Microfibril-associated glycoprotein 4 (MFAP4) is a 36 kDa extracellular matrix glycoprotein present in elastic fibre-rich tissues. MFAP4 consists of an N-terminal signal peptide, an RGD recognition site for cell surface integrin receptors, and a C-terminal fibrinogen-related domain (FReD), which constitutes the bulk of the protein. MFAP4 partakes in elastin fibre formation (elastogenesis) and in extracellular matrix organisation by protein-protein and cell-matrix interactions. MFAP4 multimerises and interacts with elastogenic proteins, including fibrillin-1 and tropoelastin, and with cells via integrins.

The presented 2D classes were collectively used for initial reference generation and subsequent 3D reconstruction using C1 point group symmetry, confirming that MFAP4 organizes as an octameric structure. Further refinement of the 3D cryo-EM map with D2 symmetry produced a 3.55 Å resolution (masked Fourier shell correlation (FSC)half-map = 0.143, Supplementary Figs. 2 and 3) structure of octameric MFAP4. Thus, the top and bottom halves of the MFAP4 octamer, defined across the central XY plane, can be described as two tetramers, each composed of two dimers with N-termini linked by C34 disulphide bonds. Within the tetrameric top and bottom halves of the MFAP4 octamer, monomers interact through intra-tetrameric interfaces, including potential salt-bridge interactions between interchain residues R105-D159 and R94-E158, hydrogen bonds between interchain residues A106-N152, G104-E158, G104-V154, and R94-E158, as well as non-bonded interchain interactions between R105-N152, G104-D159 and F103-E158. The top and bottom halves of the MFAP4 octamer associate through inter-tetrameric interfaces, including a polar non-bonded interchain interaction between N231-A200 and non-polar non-bonded interchain interactions between V196-F93, L202-L202, S204-L202. Between tetrameric halves of the MFAP4 octamer, the buried solvent-accessible surface area is 433 Å2 and is shared between 22 contacting residues (13 residues from each adjacent chain). Although the N-termini preceding Q37 are not resolved within the map model and are predicted to be disordered regions by AlphaFold2, we observed that the Q37 residues of each of the four MFAP4 molecules at the top and bottom of an octamer are positioned to extend towards each other and outwards from the macromolecular assembly. This arrangement potentially positions four integrin-binding RGD motifs at each of the poles of the MFAP4 octamer (orange residues). We noticed that S186, D191, and Q192 sidechains, as well as the backbone carbonyl group of T187 were all capable of binding Ca2+ at this position. We propose that this Ca2+ helps to push loop A182-A206 away from MFAP4’s centre of mass and towards the opposing A182-A206 loop of the other MFAP4 molecules, thus stabilising inter-tetrameric interactions between V196-F93, L202-L202, S204-L202, and N231-A200 to form octamers.

>[8x]QVSGIRGDALERFCLQQPLDCDDIYAQGYQSDGVYLIYPSGPSVPVPVFCDMTTEGGKWTVFQKRFNGSVSFFRGWNDYKLGFGRADGEYWLGLQNMHLLTLKQKYELRVDLEDFENNTAYAKYADFSISPNAVSAEEDGYTLFVAGFEDGGAGDSLSYHSGQKFSTFDRDQDLFVQNCAALSSGAFWFRSCHFANLNGFYLGGSHLSYANGINWAQWKGFYYSLKRTEMKIRRAGKPIPNPLLGLDSTRTGHHHHHHHH> SGDSSISISAIGNVDSPMIRITFQNQTEREFFLNKITDKAKSLGVNISTHPFEIKEPNMVLIKPSKYPDNKLGCYISKNKEIAINFGRTDFRDFVLSNLGVGSHLGTCPTKNETGNDTFYFHQENLSLNGPALSVN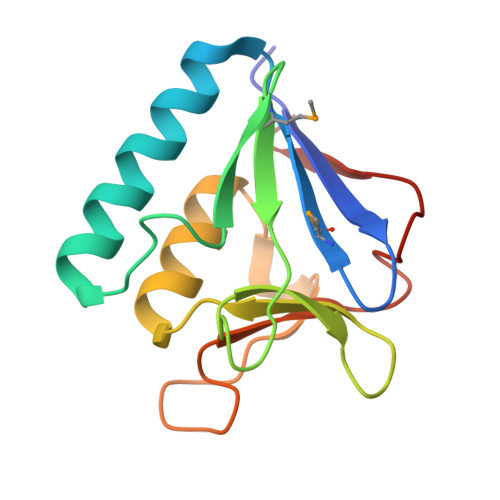TK>MVEYHIPSWDEIEDAVFSIGEALVKSNYIPDVLIAVLTGGIIPAKLLSDLLDLKVIRYIDIKFYRSVGKTESKPVIRSVYTDSLEGKKVLVVDDVADTGETLEAVSNVITMFNPAKVMTAALYLKPWSKRIPDFYYKQIDKWII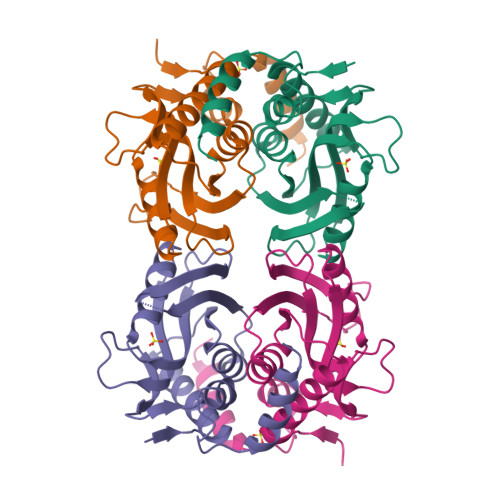FPWDKWDVVRENSNVPVDKKERFLNLYNQLLKIRK[6x]> SDWISFSHMSSDTDHFPIKSWFRCEQKAASRSYATLGDMSHPQGIYEVRAAITRLISLTRGVKCRPEQMIIGAGTQVLMQLLTELLPKEAVYAMEEPGYRRMYQLLKNAGKQVKTIMLDEKGMS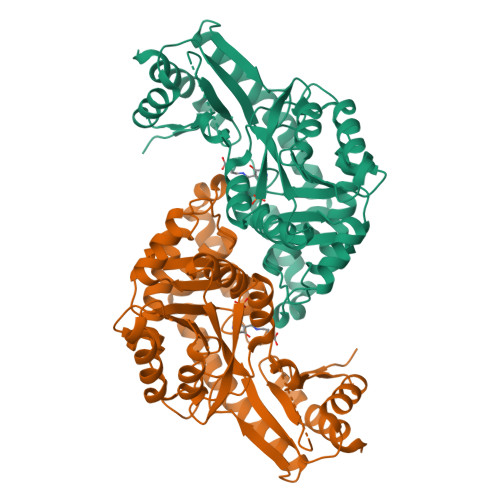IAEITRQQPDVLVTTPSHQFPSGTIMPVSRRIQLLNWAAEEPARYIIEDDYDSEFTYDVESIPALQSLDRFQNVIYMGTFSKSLLPGLRISYMVLPPELLRAYKQRGYDLQTCSSLTQLTLQEFIESGEYQKHIKKMKQHYKEKRERLITALEAEFSGEVTVKGANAGLHFVTEFDTRRTEQDILSHAAGLQLEIFGMSRFNLKENKRQTGRPTLIIGFARLKEEDIQEGVQRLFKAVYGH>[8x]SELDSENDAADIAAGTIIAGAELTFGLLQNLLYFFANVNRKCAVGVDNESGFRWQ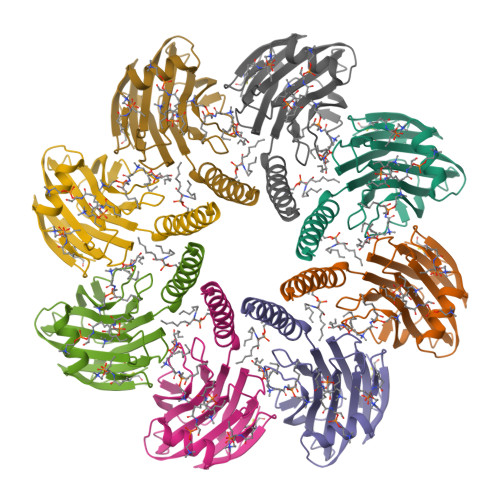EGSTYFFSGTADENLPYSVSDGYAVLYGPRKTNGPVATGVVGVLAYYIPSIGKTLAVMWSVPFDYNFYQNWWNAKLYSGNQRADYDHYVDLYYNANPFKANGWHERSLGSGLKFCGSMSSSGQATLEIHVLKESETCM The capsaicin- and heat-activated receptor, TRPV1, has served as a model for deciphering lipid modulation, which is relevant to understanding how pro-algesic agents enhance channel activity in the setting of inflammatory pain. Identification of a pocket within the TRPV1 transmembrane core has provided initial clues as to how phosphoinositide lipids bind to and regulate the channel. Here we show that this regulatory pocket in rat TRPV1 can accommodate diverse lipid species, including the inflammatory lipid lysophosphatidic acid, whose actions are determined by their specific modes of binding. We captured several states of TRPV1 ranging from channels in which the VBP is empty to those bearing different bioactive lipids, including distinct phosphoinositide species, brominated phosphoinositide analogs and a pro-algesic lipid, lysophosphatidic acid (LPA). Together, our data show how the VBP accommodates a range of bioactive lipids and how occupancy of the site corresponds to the structural status of the pore.

To determine the effect of the resident PI lipid on channel gating, we devised a protocol to eject this lipid and render the binding pocket empty. First, we used capsaicin to displace the resident lipid from detergent-solubilized channels. We then washed out the competing vanilloid followed by reconstitution of the channel into lipid nanodiscs of defined composition and devoid of phosphoinositide lipids. These samples were applied to grids held at 4 °C or 25 °C (temperatures at which TRPV1 is normally closed) and then taken forward for cryo-EM analysis. The final maps were refined using C4 symmetry and resolved to 2.9 Å and 3.7 Å for the 4 °C and 25 °C samples, respectively. In both cryo-EM structures the vanilloid pocket is, indeed, unoccupied by either a resident PI lipid or capsaicin. Interestingly, we observed that Y511 is flipped toward the binding pocket in these two structures, akin to what is seen in the agonist-bound state, demonstrating that reorientation of this fiducial side chain primarily reflects ejection of the resident lipid. We also see transition of a π-helical turn in S6 to an α-helical configuration (π–α transition), resulting in rotation of the lower half of the S6 helix by one residue. This π–α transition rotates the gating residue L679 away from the central axis with a narrowest restriction now formed by rotation of M682 into the pore. Indeed, consistent with our previous study6, the difference in the B factor of M682 compared to a nearby residue (A680) is 15.01 Å2 for data at 25 °C and 10.57 Å2 for data at 4 °C. This is substantially higher than the B factor difference in the apo state (~1 Å2), which shows that M682 is more dynamic in the α state, and thus suggesting that M682 is sufficiently malleable to pass ions in the α state.

>[4x]SYYKGQTALHIAIERRNMTLVTLLVENGADVQAAANGDFFKKTKGRPGFYFGELPLSLAACTNQLAIVKFLLQNSWQPADISARDSVGNTVLHALVEVADNTVDNTKFVTSMYNEILILGAKLHPTLKLEEITNRKGLTPLALAASSGKIGVLAYILQREIHEPECRHLSRKFTEWAYGPVHSSLYDLSCIDTCEKNSVLEVIAYSSSETPNRHDMLLVEPLNRLLQDKWDRFVKRIFYFNFFVYCLYMIIFTAAAYYRPVEGLPPYKLKNTVGDYFRVTGEILSVSGGVYFFFRGIQYFLQRRPSLKSLFVDSYSEILFFVQSLFMLVSVVLYFSQRKEYVASMVFSLAMGWTNMLYYTRGFQQMGIYAVMIEKMILRDLCRFMFVYLVFLFGFSTAVVTLIEDGKYNSLYSTCLELFKFTIGMGDLEFTENYDFKAVFIILLLAYVILTYILLLNMLIALMGETVNKIAQESKNIWKLQRAITILDTEKSFLKCMRKAFRSGKLLQVGFTPDGKDDYRWCFRVDEVNWTTWN>[6x]MYTNSDFVVIKA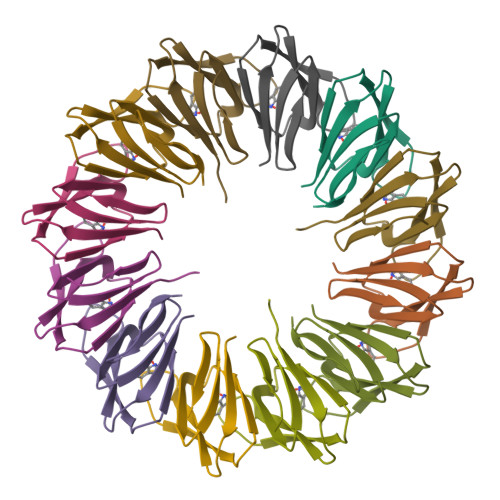LEDGVNVIGLTRGADTRFHHSEKLDKGEVLIAQFTEHTSAIKVRGKAYIQTRHGVIESEGKKAAAAAAA> GAMDPEF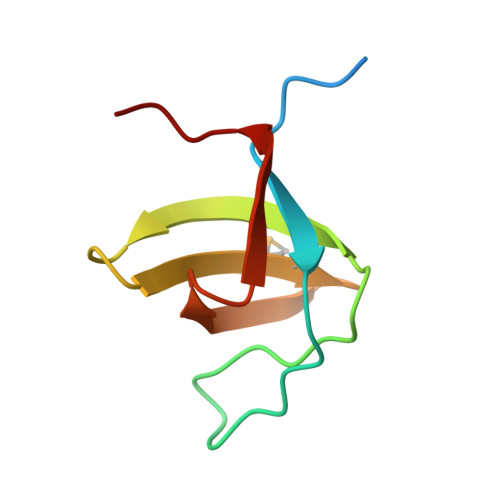MPPLDQPSCKALYDFEPENDGELGFREGDLITLTNQIDENWYEGMLHGQSGFFPLSYVQVLVPLPQ3,3-BIS(3-BROMO-4-HYDROXYPHENYL)-7-CHLORO-1H,3H-BENZO[DE]ISOCHROMEN-1-ONE | C24 H13 Br2 Cl O4 | 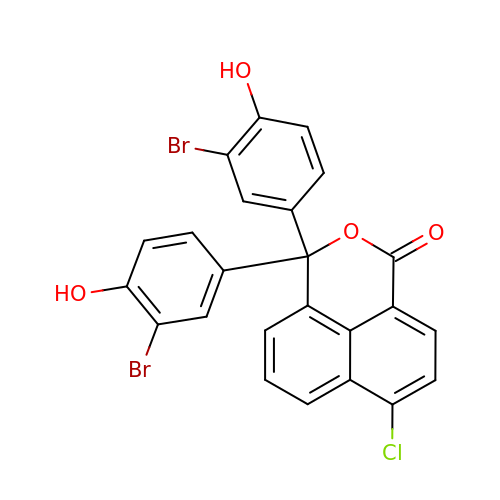GFGZCXHXQCQRFP-UHFFFAOYSA-N> MAKTQLPKLDTLSMVTMGVLMALQLVISRFSVGNNFIKVSFTFLIVALIAKWFGPWWGMLTAAVVDVIGTL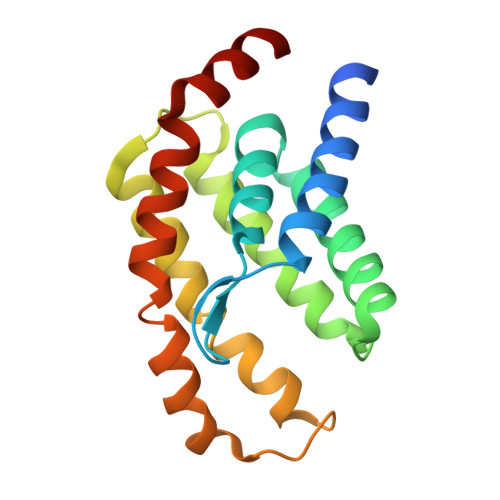MTGGPFFIGFTVSAVLGSLIYAVFLYRQPVSWWRVIGASVLIALLVNTLLNTLWVTIMYQTPFWSLLPVRALKELIVTPVQIVLVYLLLKSQVIQMIQARLNK> MGSSHHHHHHSQDPQDLNFGQVVADVLCEFLEVAVHLILYVREVYPVGIFQKRKKYNVPVQ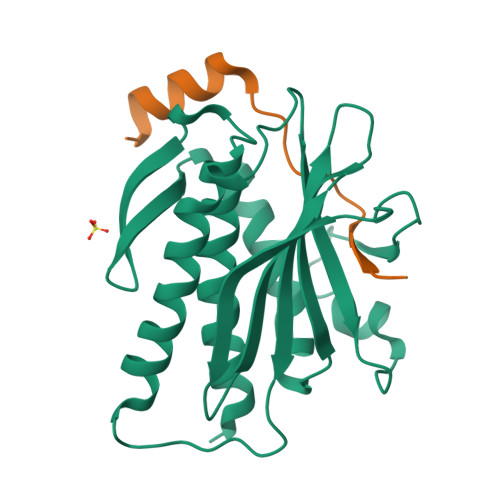MSCHPELNQYIQDTLHCVKPLLEKNDVEKVVVVILDKEHRPVEKFVFEITQPPLLSISSDSLLSHVEQLLAAFILKISVCDAVLDHNPPGCTFTVLVHTREAATRNMEKIQVIKDFPWILADEQDVHMHDPRLIPLKTMTSDILKMQLYVEERAHKGS;> MGSKLPLRPKRSPPVISEEAAEDVKQYLTI>[20x]AKLETVTLGNIGKDGKQTLVLNPRGVNPTNGVASLSQAGAVPALEKRVTVSVSQPSRNRKNYKVQVKIQNPTACTANGSCDPSVTRQAYADVTFS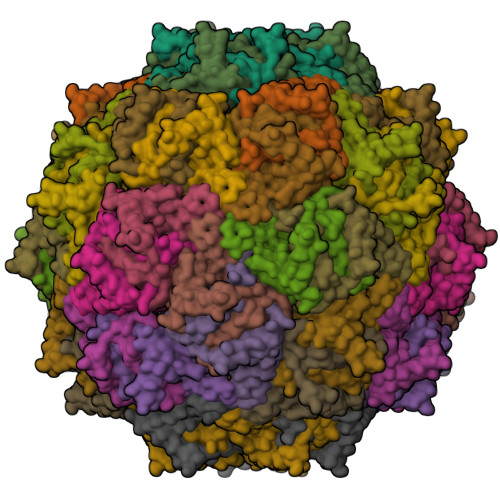FTQYSTDEERAFVRTELAALLASPLLIDAIDQLNPAY>GAADGEGRGELSPKIKAGDLESKLIVPKNNGLKITGTFLDEISHDIPHQNWGEKEWDLDFQHMKRIGIDTVIMIRSGYRKFMTYPSPYLLKKGCYMPSVDLVDMYLRLAEKYNMKFYFGLYDSGRYWDTGDLSWEIEDN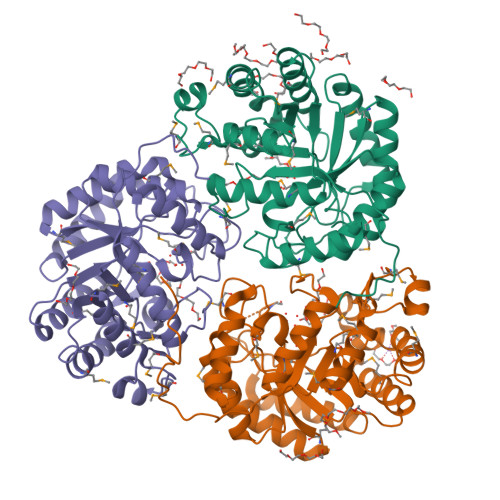KYVIDEVWKMYGEKYKSFGGWYISGEISRATKGAIDAFRAMGKQCKDISNGLPTFISPWIDGKKAIMGTGKLTREDAVSVQQHEKEWNEIFDGIHEVVDACAFQDGHIDYDELDAFFTVNKKLADKYGMQCWTNAESFDRDMPIRFLPIKFDKLRMKLEAAKRAGYDKAITFEFSHFMSPQSAYLQAGHLYDRYREYFEIK[3x]(6~{R})-~{N}-(4-chlorophenyl)-1-methyl-8-(1-methylpyrazol-4-yl)-5,6-dihydro-4~{H}-[1,2,4]triazolo[4,3-a][1]benzazepin-6-amine 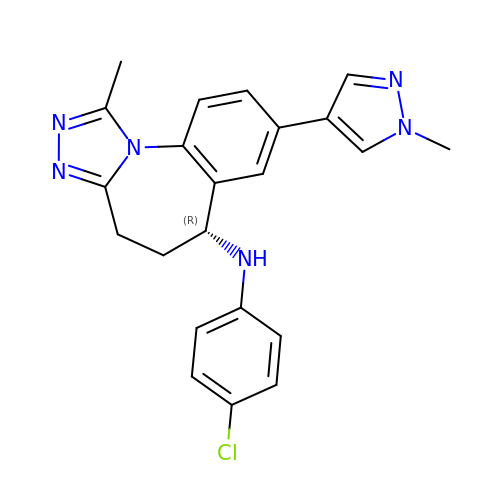| C22 H21 Cl N6 | MDRXOFSNECSECW-HXUWFJFHSA-N> GVENAEKGVTENTDATADFVAQPVYLPENQTKVAFFYDRSSPIGRFAVKSGSLESGFAPFSNKACPNSVILTPGPQFDPAYDQLRPQRLTEIWGNGNEETSEVFPLKTKQDYSFCLFSPFVYYKCDLEVTLSPHTSGAHGLLVRWCPTGTPTKPTTQVLHEVSSLSE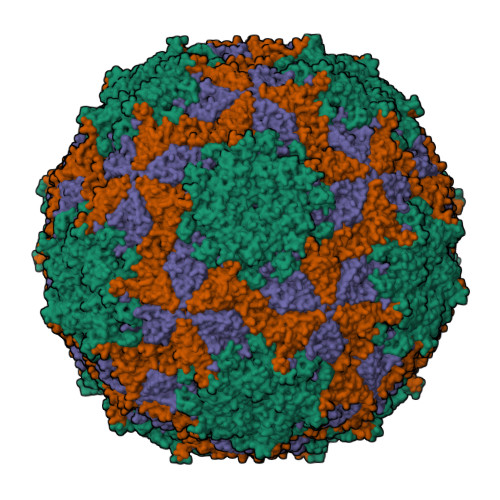GRTPQVYSAGPGTSNQISFVVPYNSPLSVLPAVWYNGHKRFDNTGDLGIAPNSDFGTLFFAGTKPDIKFTVYLRYKNMRVFCPRPTVFFPWPTSGDKIDMTPRAGVL;> DQNTEEMENLSDRVSQDTAGNTVTNTQSTVGRLVGYGTVHDGEHPASCADTASEKILAVERYYTFKVNDWTSTQKPFEYIRIPLPHVLSGEDGGVFGATLRRHYLVKTGWRVQVQCNASQFHAGSLLVFMAPEYPTLDVFAMDNRWSKDNLPNGTRTQTNRKGPFAMDHQNFWQWTLYPHQFLNLRTNTTVDLEVPYVNIAPTSSWTQHASWTLVIAVVAPLTYSTGASTSLDITASIQPVRPVFNGLRHEVLSRQ;> SPIPVTIREHAGTWYSTLPDSTVPIYGKTPVAPANYMVGEYKDFLEIAQIPTFIGNKMPNAVPYIEASNTAVKTQPLAVYQVTLSCSCLANTFLAALSRNFAQYRGSLVYTFVFTGTAMMKGKFLIAYTPPGAGKPTSRDQAMQATYAIWDLGLNSSYSFTVPFISPTHFRMVGTDQANITNVDGWVTVWQLTPLTYPPGCPTSAKILTMVSAGKDFSLKMPISPAPWSPQ;> GNSTSSDKNNSSSEGNEGVIINNFYSNQYQNSIDLSANATGSDPPKTYGQFSNLLSGAVNAFSNMLPLLA> GEKQDLEKIESDIINDWTEADDLDDALDFLF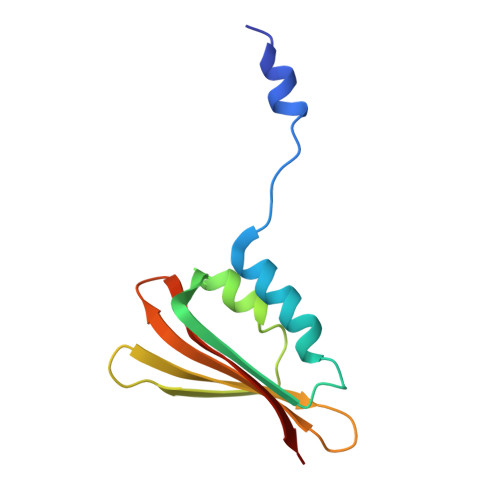MEKVSEFKIKFKDPLKVTEEEYRELLGNYDSSNSVSSNGITIDQYTYDEDDDIMYKLEFTYRKEDNKIYIYEVQGWREKKK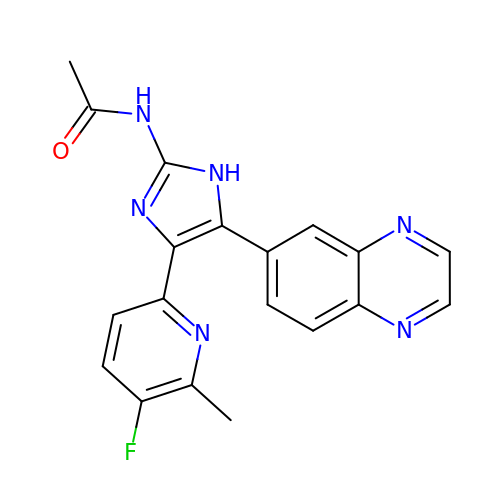N-[4-(5-fluoro-6-methylpyridin-2-yl)-5-quinoxalin-6-yl-1H-imidazol-2-yl]acetamide | C19 H15 F N6 O | TYPILNNEZPSNTI-UHFFFAOYSA-N>GSHMEEPEEPADSGQSLVPVYIYSPEYVSMCDSLA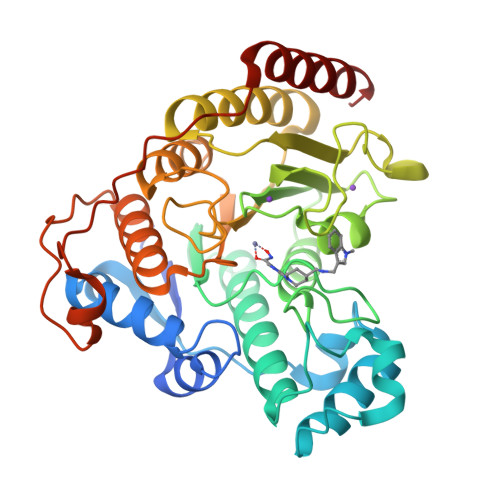KIPKRASMVHSLIEAYALHKQMRIVKPKVASMEEMATFHTDAYLQHLQKVSQEGDDDHPDSIEYGLGYDCPATEGIFDYAAAIGGATITAAQCLIDGMCKVAINWSGGWHHAKKDEASGFCYLNDAVLGILRLRRKFERILYVDLDLHHGDGVEDAFSFTSKVMTVSLHKFSPGFFPGTGDVSDVGLGKGRYYSVNVPIQDGIQDEKYYQICESVLKEVYQAFNPKAVVLQLGADTISGDRLGCFNMTPVGIGKCLKYILQWQLATLILGGGGYNLANTARCWTYLTGVILGKTLSSEIPDHEFFTAYGPDYVLEITPSCRPDRNEPHRIQQILNYIKGNLKHVV[2x]> MSKFLDRFRYFKQKGETFADGHGQLLNTNRDWEDGYRQRWQHDKIVRSTHGVNCTGSCSWKIYVKNGLVTWETQQTDYPRTRPDLPNHEPRGCPRGASYSWYLYSANRLKYPMMRKRLMKMWREAKALHSDPVEAWASIIEDADKAKSFKQARGRGGFVRSSWQEVNELIAASNVYTIKNYGPDRVAGFSPIPAMSMVSYASGARYLSLIGGTCLSFYDWYCDLPPASPQTWGEQTDVPESADWYNSSYIIAWGSNVPQTRTPDAHFFTEVRYKGTKTVAVTPDYAEIAKLCDLWLAPKQGTDAAMALAMGHVMLREFHLDNPSQYFTDYVRRYTDMPMLVMLEERDGYYAAGRMLRAADLVDALGQENNPEWKTVAFNTNGEMVAPNGSIGFRWGEKGKWNLEQRDGKTGEETELQLSLLGSQDEIAEVGFPYFGGDGTEHFNKVELENVLLHKLPVKRLQLADGSTALVTTVYDLTLANYGLERGLNDVNCATSYDDVKAYTPAWAEQITGVSRSQIIRIAREFADNADKTHGRSMIIVGAGLNHWYHLDMNYRGLINMLIFCGCVGQSGGGWAHYVGQEKLRPQTGWQPLAFALDWQRPARHMNSTSYFYNHSSQWRYETVTAEELLSPMADKSRYTGHLIDFNVRAERMGWLPSAPQLGTN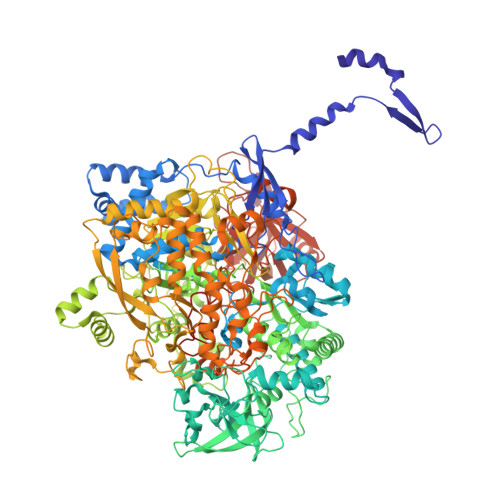PLTIAGEAEKAGMNPVDYTVKSLKEGSIRFAAEQPENGKNHPRNLFIWRSNLLGSSGKGHEFMLKYLLGTEHGIQGKDLGQQGGVKPEEVDWQDNGLEGKLDLVVTLDFRLSSTCLYSDIILPTATWYEKDDMNTSDMHPFIHPLSAAVDPAWEAKSDWEIYKAIAKKFSEVCVGHLGKETDIVTLPIQHDSAAELAQPLDVKDWKKGECDLIPGKTAPHIMVVERDYPATYERFTSIGPLMEKIGNGGKGIAWNTQSEMDLLRKLNYTKAEGPAKGQPMLNTAIDAAEMILTLAPETNGQVAVKAWAALSEFTGRDHTHLALNKEDEKIRFRDIQAQPRKIISSPTWSGLEDEHVSYNAGYTNVHELIPWRTLSGRQQLYQDHQWMRDFGESLLVYRPPIDTRSVKEVIGQKSNGNQEKALNFLTPHQKWGIHSTYSDNLLMLTLGRGGPVVWLSEADAKDLGIADNDWIEVFNSNGALTARAVVSQRVPAGMTMMYHAQERIVNLPGSEITQQRGGIHNSVTRITPKPTHMIGGYAHLAYGFNYYGTVGSNRDEFVVVRKMKNIDWLDGEGNDQVQESVK> SRMQLSEEQAAVLRAVLKGQSIFFTGSAGTGKSYLLKRILGSLPPTGTVATASTGVAACHIGGTTLHAFAGIGSGQAPLAQCVALAQRPGVRQGWLNCQRLVIDEISMVEADLFDKLEAVARAVRQQNKPFGGIQLIICGDFLQLPPVTKGSQPPRFCFQSKSWKRCVPVTLELTKVWRQADQTFISLLQAVRLGRCSDEVTRQLQATASHKVGRDGIVATRLCTHQDDVALTNERRLQELPGKVHRFEAMDSNPELASTLD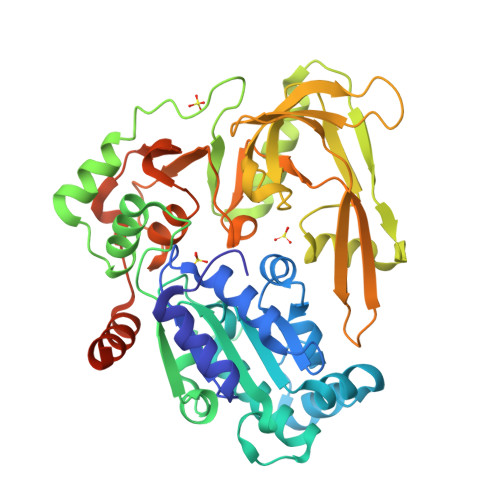AQCPVSQLLQLKLGAQVMLVKNLSVSRGLVNGARGVVVGFEAEGRGLPQVRFLCGVTEVIHADRWTVQATGGQLLSRQQLPLQLAWAMSIHKSQGMTLDCVEISLGRVFASGQAYVALSRARSLQGLRVLDFDPMAVRCDPRVLHFYATLRRGRSLSLESPDDDEAASDQENMDPIL p-coumaroyl-CoA | C30 H42 N7 O18 P3 S | 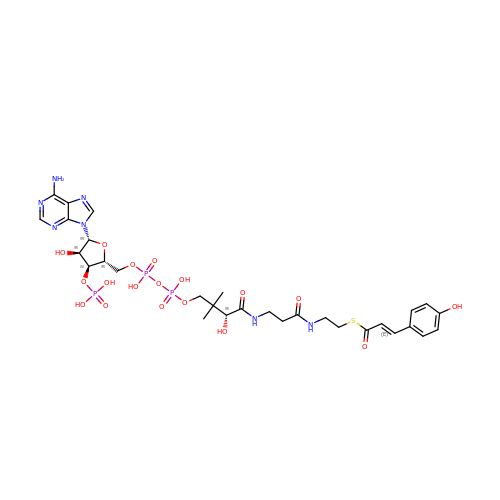DMZOKBALNZWDKI-MATMFAIHSA-N> MITIKKQEIVKLEDVLHLYQAVGW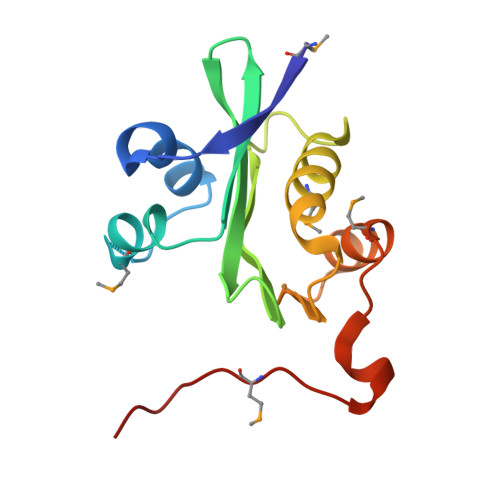TNYTHQTEMLEQALSHSLVIYLALDGDAVVGLIRLVGDGFSSVFVQDLIVLPSYQRQGIGSSLMKEALGNFKEAYQVQLATEETEKNVGFYRSMGFEILSTYDCTGMIWINREK>[3x]MKE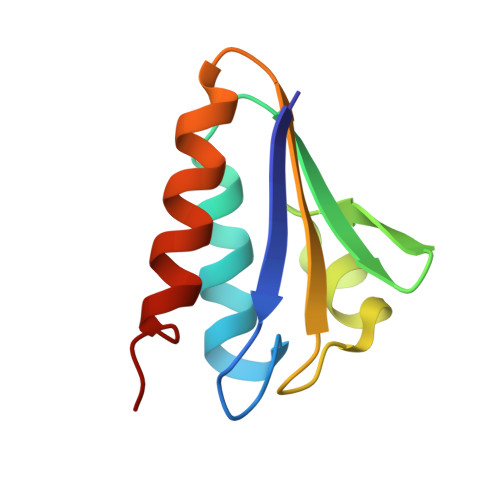VTIEIKNKTGLHARPAALFVQTASKFSSQIWVEKDNKKVNAKSIMGIMSLGVSQGNVVKLSAEGDDEEEAIKALVDLIESKFGEE Here, we present the near-atomic resolution structure of Haloferax tailed virus 1 (HFTV1), an archaeal virus thriving in extreme salinity. Through single-particle analysis, we obtained near-atomic resolution maps of DNA-filled and empty virions, enabling us to assemble full atomic models of the virus pre- and post-DNA release, including all structural protein components. The full atomic structure revealed that the virus has a length of 1350 Å and an icosahedral head with a diameter of ~600 Å. The tail has a length of 560 Å and terminates into a baseplate with three radiating TFs of ~190 Å in length.

Threefold rotational (C3) averaging focused on a single turret position produced a 2.36-Å-resolution map (flowchart S1). Turrets were found to consist of two separate proteins; a base formed of a hexamer of gp30 [turret base protein (TBP); Fig. 4], and a trimeric turret head protein (THP) gp31. The THP trimer then inserts into the TBP hexamer with a longer, 12-stranded triangular barrel, elevating the THP above the TBP. Six histidine modifications (likely phosphohistidines) are found at the hexamer-trimer interface. While all these modified histidines belong to the TBP, three directly interact with the N termini of the THP trimer via salt bridges, contributing to the stability of the interaction between the THP and TBP. Alongside three Mg2+ ions, the THP trimer includes three catalytic Zn2+ coordination sites. Analyzing the structure of the THP using DALI and National Center for Biotechnology Information (NCBI) Basic Local Alignment Search Tool (BLAST) indicated a similarity between THP and polysaccharide deacetylases from multiple species. InterProScan reports that the deacetylase-like domain encompasses residues 199 to 413, ending at the C terminus of the THP. However, a second conserved domain is also reported, corresponding to a galactose-binding domain-like superfamily (G3DSA:2.60.120.260), which spans residues 57 to 198 and makes up the second externally facing subunit of the THP.

>[3x]MTGLNPDGLGRTAAFSNTSAESVSAVDATIDRLYAQDRIEIPTDSRQLFSTRGTVLRNFEDLSGWTANIGSLSAETSDVYVGSQSARLTASSSAVDIRYSFGTAQDFTGKGFSMALKRIDVSGSSDSTPIKIRLVDGNTNYRTFSARCRPGGGDEWGRRDFGFESEDTGFDVTNVQTMTVTTNSRSSIDILVDDIRVVDSSGTGQVIVTIDDVHTGDKTAAEVFGRYGIPIGLAANAKFLDQSSSKLTTQEFKDLLAKPHVYAVNHGYNHYDYGSYSIDEIEDDVIRGKYELQDLGVREPNINHYVYPSGNYAQESIDMLSNYHVMSWGTGAESFDALTPNQLTSPWHNLRCSFDSGTAEAEQAVNDAATYNQTAHIYFHSDNVTQSEMESVAQTINSADVTPITLMDFYNQQ;>MTDTIVNVQGSFFSASASGVADTESLLIDPQDAKFGAIEIHNIAHGGSVDVELLTSSDDTELVEDAAVTLDSFTGEGISQGNQIEASDNTNTYIRITNTSGGAIDIIATGREVSQ[6x]>MLEANVYDNFNPNYYNISDFSMPNGKKEKRGLPIPKARCQVI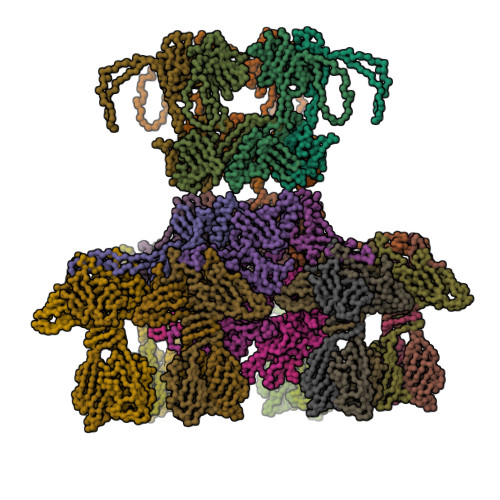NYELWETGYLYTSSATLTVSVEVGDIVQILFPEVVPIEEALGKKKKLNLDMVYLVTDVDESNKATLKNYFWAMIESLDVPNAITKTTNFAIIDYLIDPNKNNLMSYGYFFNSSIFAGKATINRKAETSSAHDVAKRIFSKVQFQPTTTIQHAPSETDPRNLLFINFASRNWNRKRITTRVDIKQSVTMDTETIVERSAYNFAVVFVKNKATDDYTDPPKMYIAKNNGDVIDYSTYHGDGTDLPDVRTAKTLFYDRDDHGNPPELSTIKVEISPSTIVTRLIFNQNELLPLYVNDLVDIWYEGKLYSGYIADRVKTEFNDRLIFVESGDKPNVI[3x];>[12x]MVRQYKIHTNLDGTDDKVWDVTNGKVRFYQPSNLGLQSTNNIWQSNGIGVMGTRSITQPQIEFKLETFGESLEENYQLMKDFVNDILSKKFVTLEYQTEIFQVYADLALADVTKTEGYGKNGTFSEKITFDIITKWYTYENLTFDKIQNGKVIAGMSKIYGGTAPGNYKYIKGTSYTYYGESDIDRLSRWDIKEEIFSFMGILYPKLPKTPAGVRFLDDIGNEYTAIVFKTEQVQDYILINTDVNDETYQGWKGTTALNLFPVMDFERYRTRIIEKGQMELINLSKAEFKIKRKADFV;>MTIKNFTFFSPNSTEFPVGSNNDGKLYMMLTGMDYRTIRRKDWSSPLNTALNVQYTNTSIIAGGRYFELLNETVALKGDSVNYIHANIDLTQTANPVSLSAETANNSNGVDINNGSGVLKVCFDIVTTSGTGVTSTKPIVQTSTLDSISVNDMTVSGSIDVPVQTLTVEAGNGLQLQLTKKNNDLVIVRFFGSVSNIQKGWNMSGTWVDRPFRPAAVQSLVGHFAGRDTSFHIDINPNGSITWWGANIDKTPIATRGNGSYFIK[18x]>GPLGSYGDAIPEVKAILEAKNEEELVTFTSRWSAEERKELRTQFQDTTGLEFIAFLKKCIKNGPYEDVMALGWDCNISARVNVIKKAMKNVNDFRAIHDVVLIATPDERLKLAQAYKEKTGNDLLQDFVDQIPLTSAASYLCHLAIRENRTPRGSVASDAEVLKHNLIDADEPDHEAVVRLIITSTADEYKEINHRFEVLTGKSVQEAIETRYADKENARGLCIAHYYNLAPARAVAYAFHSAVETQNDDMAYEQAARITGLFHDLHKFAWVHY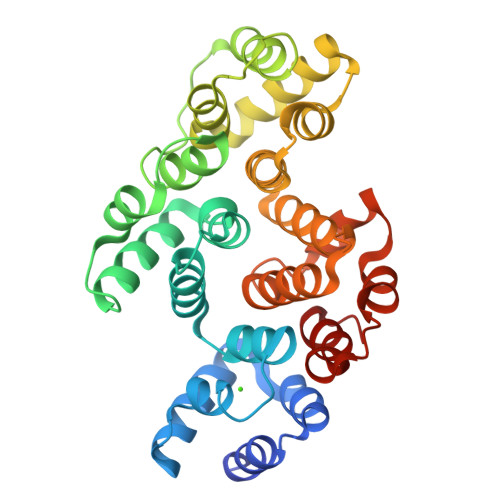ACWGVMRDDILSRFQSKEANKVNFRDACLMFWKLAK[4x]> 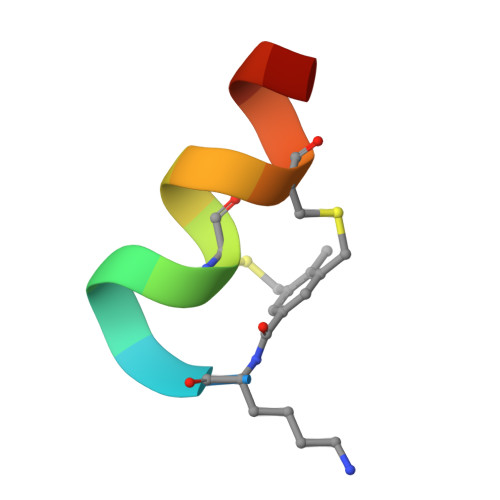XKKLLKCLKCLLKX>[6x]ERVAVVGVPMDLGANRRGVDMGPSALRYARLLEQLEDLGYTVEDLGDVPVSLARASRRRGRGLAYLEEIRAAALVLKERLAALPEGVFPIVLGGDHSLSMGSVAGAARGRRVGV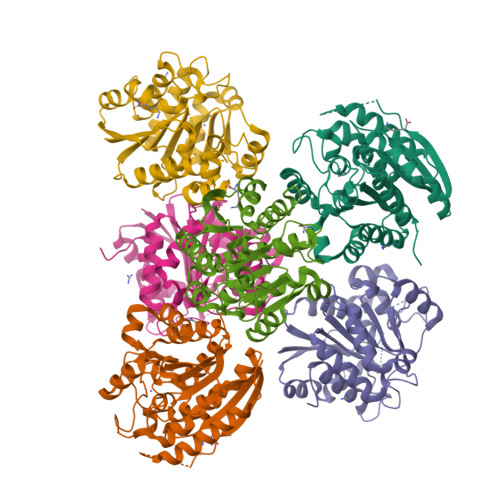VWVDAHADFNTPETSPSGNVHGMPLAVLSGLGHPRLTEVFRAVDPKDVVLVGVRSLDPGEKRLLKEAGVRVYTMHEVDRLGVARIAEEVLKHLQGLPLHVSLDADVLDPTLAPGVGTPVPGGLTYREAHLLMEILAESGRVQSLDLVEVNPILDERNRTAEMLVGLALSLLGKRIF> AQKTFKVTADSGIHARPATVLVQTAS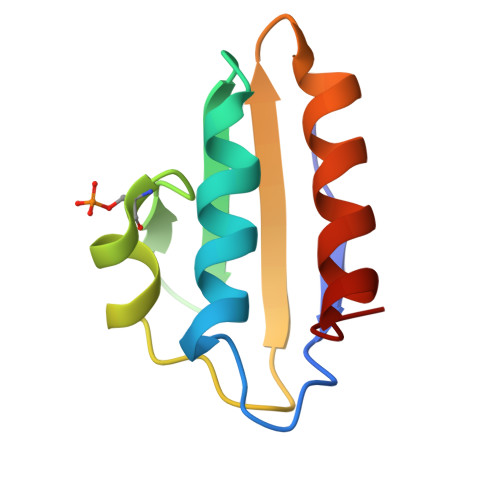KYDADVNLEYNGKTVNLKSIMGVMSLGIAKGAEITISASGADENDALNALEETMKSEGLGE> SMCKPITGTINDLNQQVWTLQGQNLVAVPRSDSVTPVTVAVITCKYPEALEQGRGDPIYLGIQNPEMCLYCEKVGEQPTLQLKEQKIMDLYGQPEPVKPFLFYRAKTGRTSTL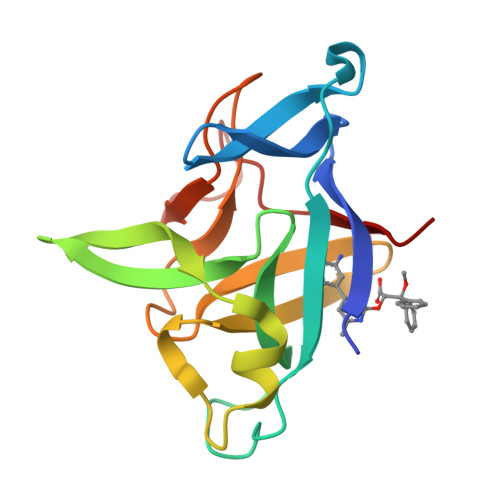ESVAFPDWFIASSKRDQPIILTSELGKSYNTAFELNIND>GPLGSHMSTESNDGVSETLLAWRHIDFWTSEHNPDLNATLSDPCTQNDITHAEEDLEVSFPNPVKASFKIHDGQEDLESMTGTSGLFYGFQLMTLDQVVAMTQAWRNVAKNLNKRSPDQKSIPPNAVQPVYAHPAWIPLITDNAGNHIGVDLAPGPNGKYAQIITFGRDFDTKFVIAENWGEFLLSFANDLEAGNWYLVDDNDDYFSGDGELVFRDKKSNGPIQDYFEVLKRRTW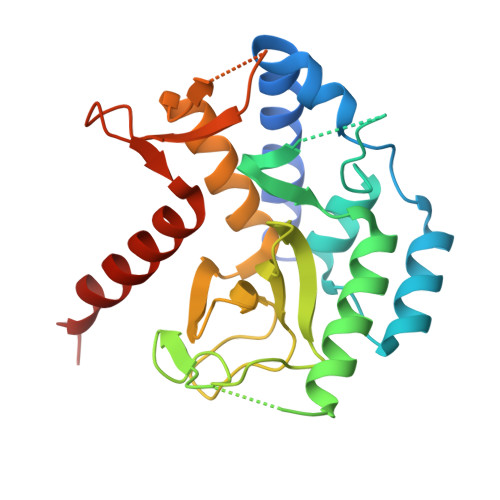IKYQLERPHRD[2x]> ELQAIHEKVKTEHAALSTEVVHL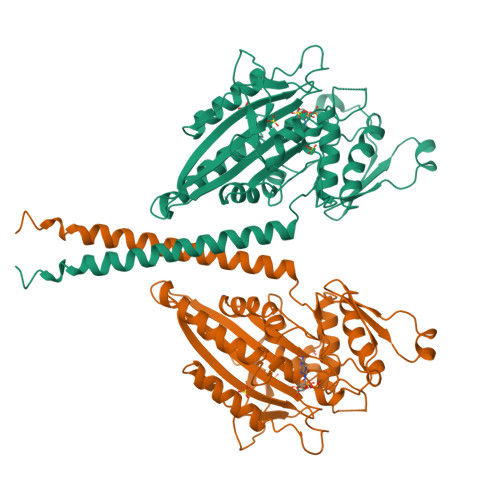RQRTEELLRCNEQQAAELETCKEQLFQSNMERKELHNTVMDLRGNIRVFCRIRPPLESEENRMCCTWTYHDESTVELQSIDAQAKSKMGQQIFSFDQVFHPLSSQSDIFEMVSPLIQSALDGYNICIFAYGQTGSGKTYTMDGVPESVGVIPRTVDLLFDSIRGYRNLGWEYEIKATFLEIYNEVLYDLLSNEQKDMEIRMAKNNKNDIYVSNITEETVLDPNHLRHLMHTAKMNRATASTAGNERSSRSHAVTKLELIGRHAEKQEISVGSINLVDLAGSESPKTSTRMTETKNINRSLSELTNVILALLQKQDHIPYRNSKLTHLLMPSLGGNSKTLMFINVSPFQDCFQESVKSLRFAASVNSCKMTKAKRNRYLNNSVANSSTQSNNSGSFDK>MSFFHASQRDALNQSLAEVQGQINVSFEFFPPRTSEMEQTLWNSIDRLSSLKPKFVSVTYGANSGERDRTHSIIKGIKDRTGLEAAPHLTCIDATPDELRTIARDYWNNGIRHIVALRGDLPPGSGKPE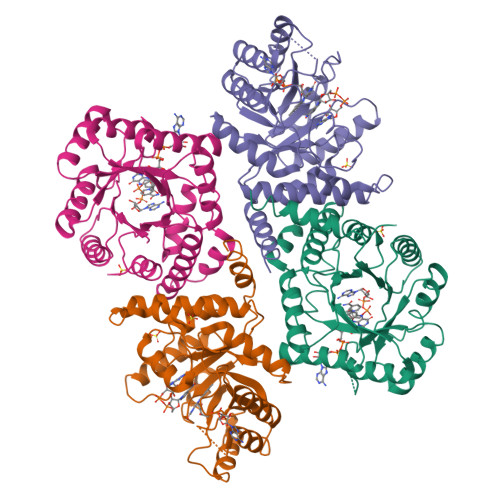MYASDLVTLLKEVADFDISVAAYPEVHPEAKSAQADLLNLKRKVDAGANRAITQFFFDVESYLRFRDRCVSAGIDVEIIPGILPVSNFKQAKKFADMTNVRIPAWMAQMFDGLDDDAETRKLVGANIAMDMVKILSREGVKDFHFYTLNRAEMSYAICHTLGVRPGLLEHHHHHH[3x]> HHHHHHMIVL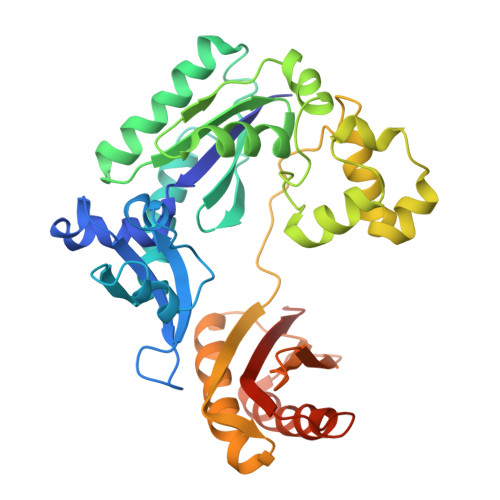FVDFDYFYAQVEEVLNPSLKGKPVVVCVFSGRFEDSGAVATANYEARKFGVKAGIPIVEAKKILPNAVYLPMRKEVYQQVSSRIMNLLREYSEKIEIASIDEAYLDISDKVRDYREAYNLGLEIKNKILEKEKITVTVGISKNKVFAKIAADMAKPNGIKVIDDEEVKRLIRELDIADVPGIGNITAEKLKKLGINKLVDTLSIEFDKLKGMIGEAKARYLISLARDEYNEPIRTRVRKSIGRIVTMKRNSRNLEEIKPYLFRAIEESYYKLDKRIPKAIHVVAVTEDLDIVSRGRTFPHGISKETAYSESVKLLQKILEEDERKIRRIGVRFSKFIEAIGLDKFFDT> DLSLE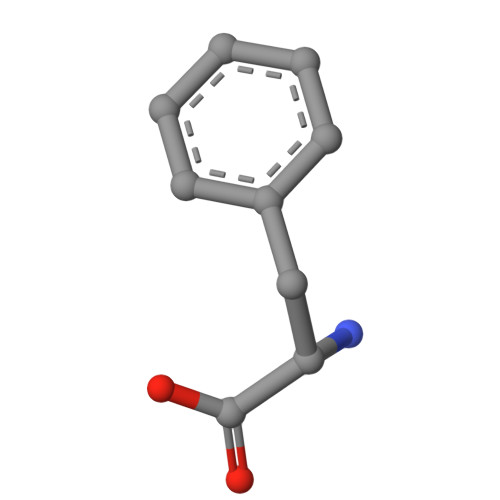DF>[4x]MGLGRQSLNIMTFSGQELTAIIKMAKSMVMADGKIKPAEIAVMTREFMRFGILQDQVDLLLKASDSIEASQAVALIARMDEERKKYVA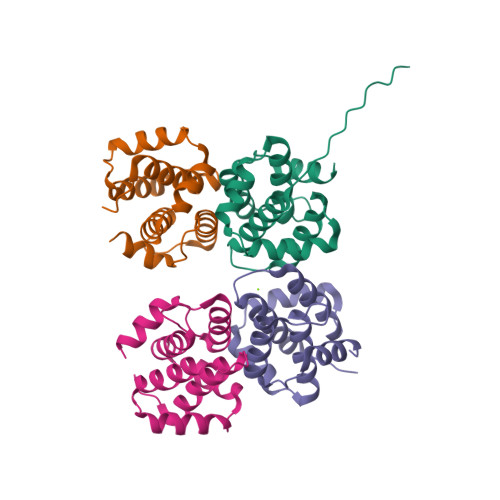SYLGVIMASDGDIDDNELALWTLISTLCGLPTMTVMEAINNMKNL>MGYQKIQVPATGDKITVNADMSLS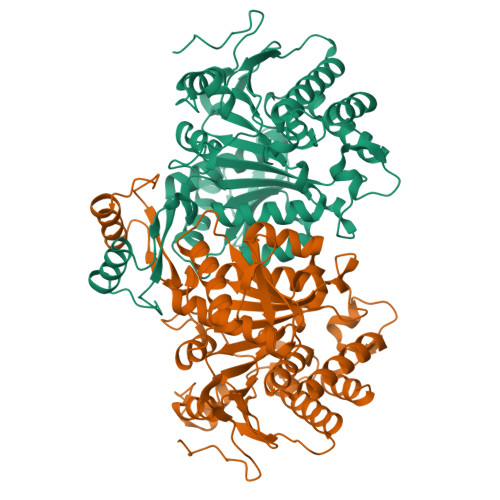VPKNPIIPFIEGDGIGVDISPVMIKVVDAAVEKAYKGERKIAWMEVYAGEKATQVYDQDTWLPQETLDAVRDYVVSIKGPLTTPVGGGIRSLNVALRQQLDLYVCQRPVRWFEGVPSPVKKPGDVDMVIFRENSEDIYAGVEWKAGSPEAEKVIKFLTEEMGVKKIRFTENCGIGIKPVSQEGTKRLVRKALQYAVDNDRSSVTLVHKGNIMKFTEGAFKDWGYEVARDEFGAELLDGGPWMQFKNPKTGKNVVVKDVIADAMLQQILLRPAEYDVIATLNLNGDYLSDALAAEVGGIGIAPGANLSDSVAMFEATHGTAPKYAGQDKVNPGSLILSAEMMLRHMGWTEAADLIIKGTNGAIAAKTVTYDFERLMDGATLLSCSEFGDAMIAKM[4x]> SPILKKIFIESPSYAPNAFTFDSTDKGFYTSVQDGRVIKYEGPNSGFTDFAYASPFWNKAFCENSTDPEKRPLCGRTYDISYDYKNSQMYIVDGHYHLCVVGKEGGYATQLATSVQGVPFKWLYAVTVDQRTGIVYFTDVSSIHDDSPEGVEEIMNTSDRTGRLMKYDPSTKETTLLLKELHVPGGAEISADGSFVVVAEFLSNRIVKYWLEGPKKGSAEFLVTIPNPGNIKRNSDGHFWVSSSEELDGGQHGRVVSRGIKFDGFGNILQVIPLPPPYEGEHFEQIQEHDGLLYIGS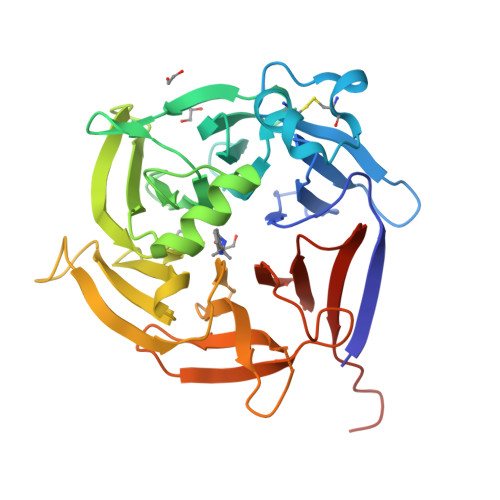LFHSSVGILVYDDHDNKGNSYVSS> MENKYSRLQISIHWLVFLLVIAAYCAMEFRGFFPRSDRPLINMIHVSCGISILVLMVVRLLLRLKYPTPPIIPKPKPMMTGLAHLGHLVIYLLFIALPVIGLVMMYNRGNPWFAFGLTMPYASEANFERVDSLKSWHETLANLGYFVIGLHA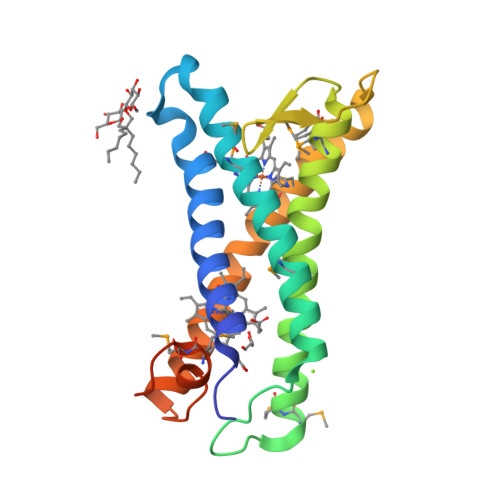AAALAHHYFWKDNTLLRMMPRKRSSVPGSHHHHHHHH> GNEWEDEQYEQYVSFKAPIASGSDGVTTIYVRYKDNGKVTYQLPIIVSGSTVNSQDRDIHIAVDKDTLKTLNIERFSLYRPELWYTEMEEDKYEFPETVHIPAGSCVELLNIDFNLQDIDMLEKWVLPLTIVDDGSYAYQSHPRKNYAKALLKVVPFNNYSGSYTASSMKVYTYINGKP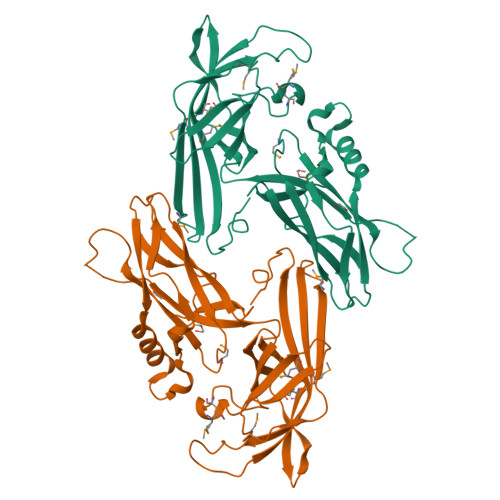DTNARTTDKRTGYVVDNNSIFFYAGLINEDMDKDMRKKYKINVHFKEDGTLDMKQDDPSNEMEFELIGTPTYSSTSVMDATRPYLERRYVQIMFEYDFQDFTYGGSGTEVIPIKYRVAGSMTLLRNINTQIPDEDQQIEW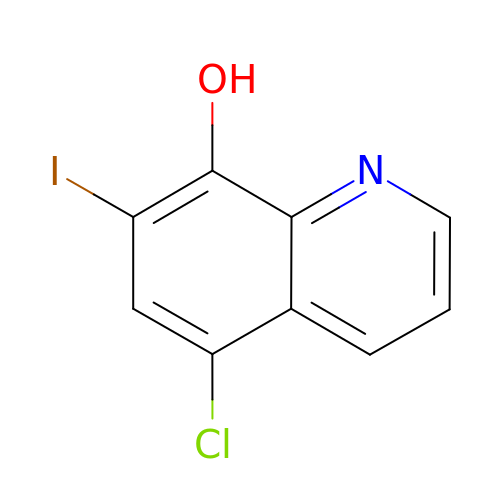5-chloro-7-iodoquinolin-8-ol | C9 H5 Cl I N O | QCDFBFJGMNKBDO-UHFFFAOYSA-N4-bromo-N'-[(1E)-(3,5-dibromo-2,4-dihydroxyphenyl)methylidene]benzohydrazide 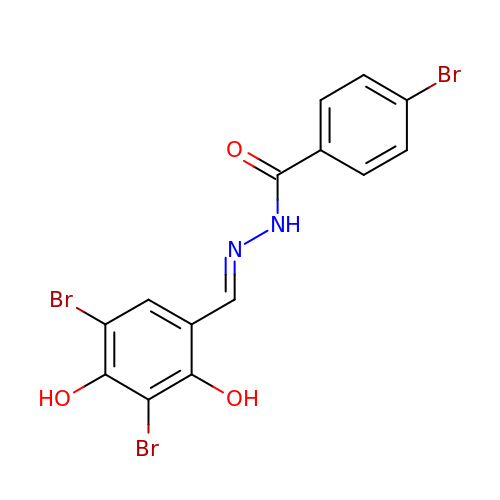| C14 H9 Br3 N2 O3 | HKNUDJDAVYPTGD-NGYBGAFCSA-N> AMAVKVAINGFGRIGRCVARIILERNDIELVAINDTTDIELTKYLFKYDTVHGEFKGSVDSEGDDLVVNGKKIKVFKSRNVKDLDFAKHGAQIVLECTGAHLTMAKCQEFIDMGVQKVIMSAPAKDDTPTYVLGVNSELYKGESIISNASCTTNCLGPVCRVLQDNFGIEKGLMTTIHAYTNGQSIIDAKAKDKRRSRAAAQNIIPTSTGAAKAMKLVMPE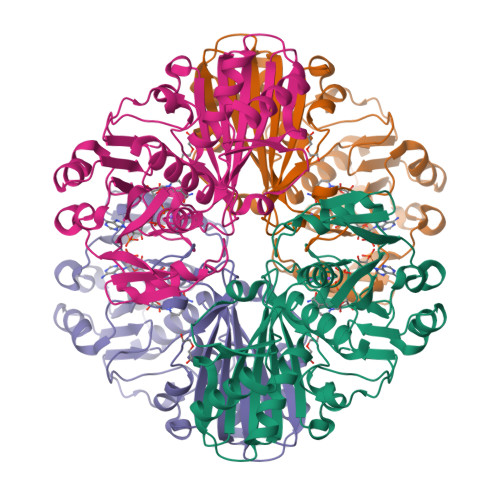LNGKLHGQSMRVPVIDVSSVDLTAQLSRKVSKDEINEAFRKAAATNLKGILMVDDDERVSSDFITCSYGAIVASDLTQVIADDFIKVIAWYDNEWGYSSRLVDMAVYIANKA>MHHHHHHGSEEQEKALNFGII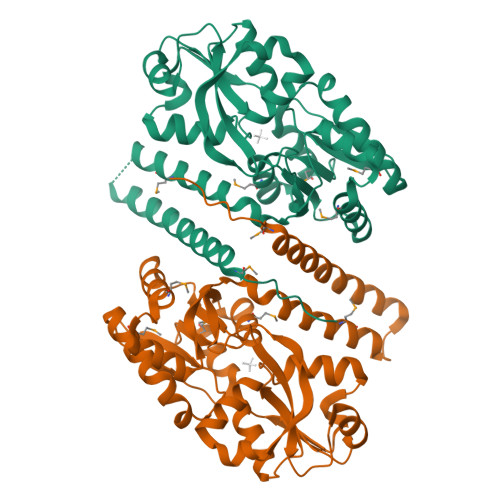STESQQNLKPQWTPFLQDMEKKLGVKVNAFFAPDYAGIIQGMRFNKVDIAWYGNLSAMEAVDRANGQVFAQTVAADGSPGYWSVLIVNKDSPINNLNDLLAKRKDLTFGNGDPNSTSGFLVPGYYVFAKNNISASDFKRTVNAGHETNALAVANKQVDVATNNTENLDKLKTSAPEKLKELKVIWKSPLIPGDPIVWRKNLSETTKDKIYDFFMNYGKTPEEKAVLERLGWAPFRASSDLQLVPIRQLALFKEMQSVKDNKGLNEQDKLAKTTAIQAQLDDLDRLNNALSAMSSVSKAVQ[2x]> SAIRG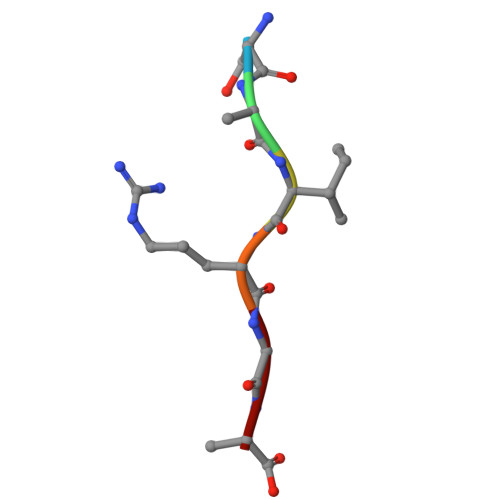A>[2x]PKFPRVKNWEVGSITYDTLSAQAQQDGPCTPRRCLGSLVFPRKLQGRPSPGPPAPEQLLSQARDFINQYYSSIKRSGSQAHEQRLQEVEAEVAATGTYQLRESELVFGAKQAWRNAPRCVGRIQWGKLQVFDARDCRSAQEMFTYICNHIKYATNRGNLRSAITVFPQR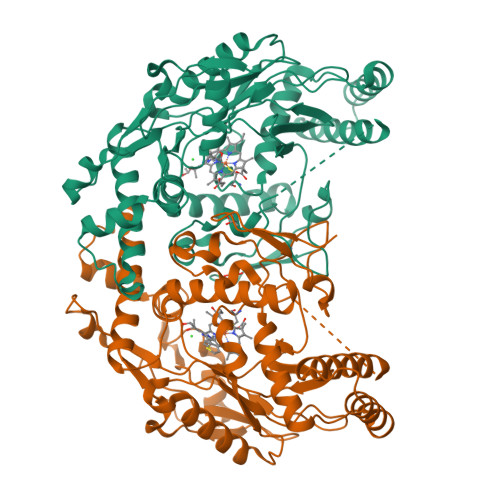CPGRGDFRIWNSQLVRYAGYRQQDGSVRGDPANVEITELCIQHGWTPGNGRFDVLPLLLQAPDEPPELFLLPPELVLEVPLEHPTLEWFAALGLRWYALPAVSNMLLEIGGLEFPAAPFSGWYMSTEIGTRNLCDPHRYNILEDVAVCMDLDTRTTSSLWKDKAAVEINVAVLHSYQLAKVTIVDHHAATASFMKHLENEQKARGGCPADWAWIVPPISGSLTPVFHQEMVNYFLSPAFRYQPDPWKGSAAKGTGITR> RPPNIVLIFADDLGYGDLGCYGHPSSTTPNLDQLAAGGLRFTDFYVPVSLATPSRAALLTGR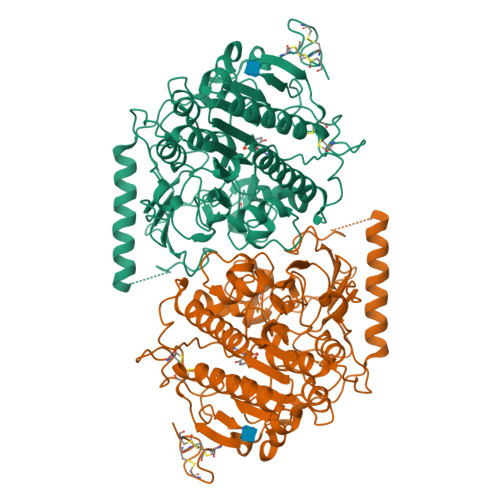LPVRMGMYPGVLVPSSRGGLPLEEVTVAEVLAARGYLTGMAGKWHLGVGPEGAFLPPHQGFHRFLGIPYSHDQGPCQNLTCFPPATPCDGGCDQGLVPIPLLANLSVEAQPPWLPGLEARYMAFAHDLMADAQRQDRPFFLYYASHHTHYPQFSGQSFAERSGRGPFGDSLMELDAAVGTLMTAIGDLGLLEETLVIFTADNGPETMRMSRGGCSGLLRCGKGTTYEGGVREPALAFWPGHIAPGVTHELASSLDLLPTLAALAGAPLPNVTLDGFDLSPLLLGTGKSPRQSLFFYPSYPDEVRGVFAVRTGKYKAHFFTQGSAHSDTTADPACHASSSLTAHEPPLLYDLSKDPGENYNLLGGVAGATPEVLQALKQLQLLKAQLDAAVTFGPSQVARGEDPALQICCHPGCTPRPACCHCPDPHA> MEVTVPDALKDRIALKKTARQLNIVYFLGSDTEPVPDYERRLSELLLYLQQFYGKEMQRHGYGARSFGLDIKSPGRVNIIEYKAKNPAAHYPYENGGGWKAAQELDEFFKAHPDRKKSQHTLIIMPTWNDEKNGPDNPGGVPFYGMGRNCFALDYPAFDIKHLGQKTREGRLLTKWYGGMAHELGHGLNLPHN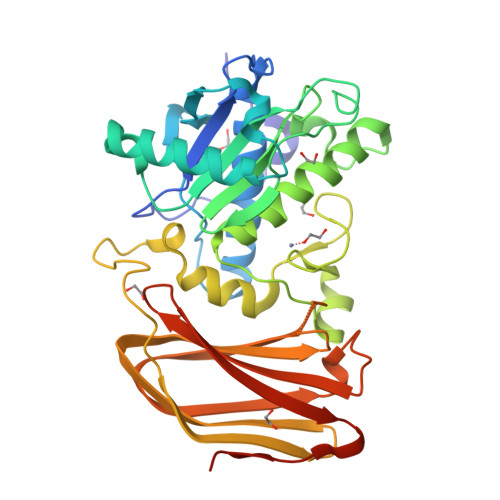HQTASDGKKYGTALMGSGNYTFGTSPTFLTPASCALLDACEVFSVTPSQQFYEGKPEVEVGDVAISFKGDQILVSGNYKSPQTVKALNVYIQDPPYAVNQDYDAVSFSRRLGKKSGKFSMKIDKKELEGLNNNEFRISLMFILANGLHMQKHFTFHWDALQDYRDGSKSGSGHHHHHH E. coli clinical isolates express the FimH adhesin, which consists of a mannose-specific lectin domain connected via a pilin domain to the tip of type 1 pili. The FimH lectin binds specifically to mannose moieties displayed on glycoproteins at the luminal surface of epithelial cells. Mannose binds in a deep and polar pocket at the N-terminal end of FimH, in which the amino acids Phe1, Asn46, Asp47, Asp54, Gln133, Asn135, Asp140 and Phe142 create a dense network of 12 hydrogen bonds with each hydroxyl group of the pyran­ose ring except that at the α-anomeric position of mannose. The interaction of the aglycones with the tyrosine gate formed by two tyrosines (Tyr48 and Tyr137) at the entrance to the FimH binding site contributes significantly to their affinity, for example with a 400-fold increase for HM compared with α-d-manno­pyranoside.

In this study, novel crystal structures of tyrosine-gate mutants of FimH, ligand-free or in complex with heptyl α-d-O-mannopyranoside or 4-biphenyl α-d-O-mannopyranoside, are combined with quantum-mechanical calculations and molecular-dynamics simulations. As no crystal structures carrying either the Y48A or Y137A mutation were available for BF, we generated all MD simulations from the WT structures after introducing the mutation in silico (see §2.11). In wild-type FimH, the mannosides exhibit largely enthalpy-driven binding, in agreement with previously reported results for other monomannoside and oligomannoside derivatives and for a series of biphenyl α-d-mannosides. The lack of the Tyr137 side chain can thus not be compensated for, probably because of its larger distance from the mannose. It has been documented that the presence of the Tyr48 side chain hinders the fit of phenyl α-d-mannosidic compounds into the binding site, however with an almost perfect enthalpy–entropy compensation. The steric hindrance by Tyr48 renders the binding highly dynamic, whereby the aromatic ligand seeks multiple stacking modes predominantly with the two tyrosines, thus including Tyr137. In contrast to HM, the flexibility of BF is almost not restricted in the WT binding site and also not in the Y137A mutant.

>[8x]FACKTANGTAIPIGGGSANVYVNLAPVVNVGQNLVVDLSTQIFCHNDYPETITDYVTLQRGSAYGGVLSNFSGTVKYSGSSYPFPTTSETPRVVYNSRTDKPWPVALYLTPVSSAGGVAIKAGSLIAVLILRQTNNYNSDDFQFVWNIYANNDVVVPT> HHHHHHVPAFLTKLWTLVSDPDTDALICWSPSGNSFHVFDQGQFAKEVLPKYFKHNNMASFVRQLNMYGFRKVVHIEQGGLVKPERDDTEFQHPCFL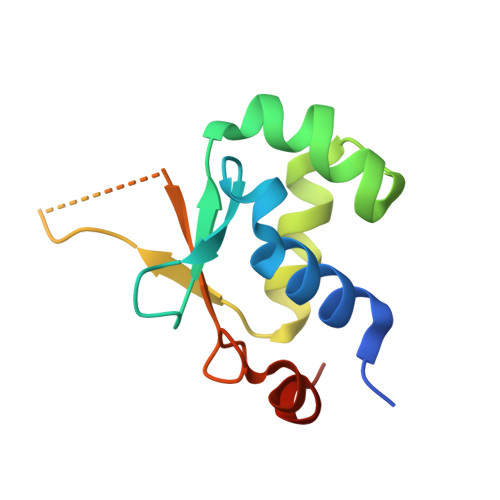RGQEQLLENIKRKVT>[2x]MAHHHHHHSAALEVLFQGPGGHLLGNRYGKIENGKLNIYSLADNSLIKTVEAGPWENMAYSMDSNSINNIDGYISYTGWYRPYGTSQDGKTWYPTTVADWRPILMYVWPSKDVQAKFIQYFVNHGYENSNYGLTTGSVKDLSENTASIKLNEVAQNLRYVIEQHIVAAKSTSQLANDINNFITTIPELSASSELPYGQVIFVNNDNTSYADSKYRLMSRTINNQTGNDNDNSDNGYEFLTGIDIDNSNPVVQAENLNWEYFLLNYGKLMGYNPDGNFDGFRIDAADHIDADVLDQTGQLMDDMYHMKGNPQNANNHLSYNEGYRSSA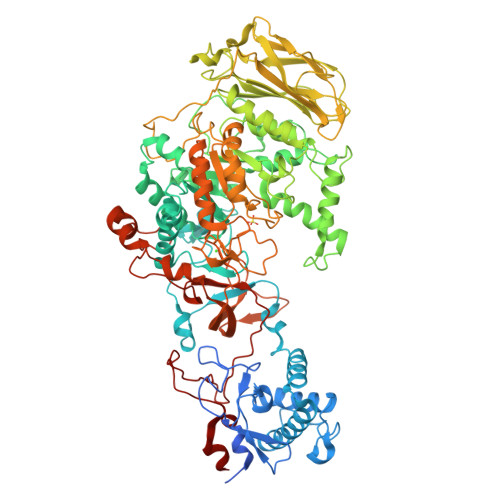ARMLNKKGNPQLYMDYVGSTLGNVLGRANNRDTISNLVTGSIVNRQNDVTENEATPNWSYVTNHDSRANLINGLISKDHPGAYKAEYANQAWQEFYADQKKTDKQYAQYNVPAQYAILLSNKDTVPQIYYGDLYNETAQYMQEKSIYYDAITTLMKARKQFVSGGQTMTKLSDNLIASVRYGKGVTNANSEGTDSLSRTSGMAVIVGNNPQMAEQTISINMGRAHANEQYRNLLDTTDNGLTYNADGAENPETLTTDDNGILKVTVKGYSNPYVSGYLGVWVPVVSGNQDVTTNAATVSADSNKIFESNAALDSHMIYQDFSLYQPEPTSTENHAYNTIAQNAELFNNLGITDFWMAPPYTQYSESRYNDGYSVTDRYNLGTNANPTKYGSGEELANAIAALHSAGLKVQVDIVMNQMIGLPGQEAVTVTRADNRGIQTYVNGKTYANQMYFAYTTGGGNGQETYGGKYLSELQSKYPDLFTTRAISTGVAPDPTTRITKWSAKYENGTSLQNIGIGLAVKLPNGEYAYLRSSDNKAFNTTLPETMSSADYYAN>ASMTGGQQMGAPITAYAQQTRGLLGCIITSLTGRDKNQVEGEVQIVSTATQTFLATCINGVCWTVYHGAGTRTIASPKGPVIQMYTNVDQDLVGWPAPQGSRSLTPCTCGSSDLYLVTRHADVIPVRRRGDSRGSLLSPRPISYLKGSSGGPLLCPAGHAVGLFRAAVCTRGVAKAVDFIPVENLETTMRSGSHHHHHH[2x];>KKGSVVIVGRIVLSGK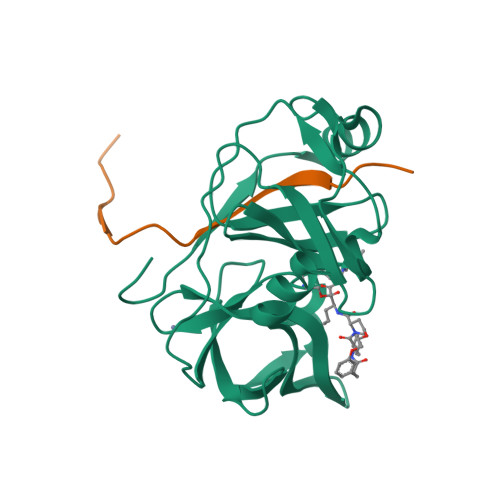PAIIPKK[2x]>AAGVAAWLPFARAAAIGWMPVASGPMPAPPRQERKRTQDALIVLNVSGTRFQTWQDTLERYPDTLLGSSERDFFYHPETQQYFFDRDPDIFRHILNFYRTGKLHYPRHECISAYDEELAFFGLIPEIIGDCCYEEYKDRRRENAERLQDDADTDTAGESALPTMTARQRVWRAFENPHTSTMALVFYYVTGFFIAVSVIANVVETVPCGSSPGHIKELPCGERYAVAFFCLDTACVMIFTVEYLLRLAAAPSRYRFVRSVMSIIDVVAILPYYIGLVMTDNEDVSGAFVTLRVFRVFRIFKFSRHSQGLRILGYTLKSCASELGFLLFSLTMAIIIFATVMFYAEKGSSASKFTSIPAAFWYTIVTMTTLGYGDMVPKTIAGKIFGSICSLSGVLVIALPVPVIVSNFSRIYHQNQRADKRRAQKKARLARIRAAKSGSANAYMQSKRSGLLSNQLQSSEDEQAFVSKSGSSFETQHHHLLHCLEKTTNHEFVD[4x];>[2x]PEGLEQLEAQTNFTKRELQVLYRGFKNECPSGVVNEDTFKQIYAQFFPHGDASTYAHYLFNAFDTTQTGSVKFEDFVTALSILLRGTVHEKLRWTFNLYDINKDGYINKEEMMDIVKAIYDMMGKYTYPVLKEDTPRQHVDVFFQKMDKNKDGIVTLDEFLESCQEDDNIMRSLQLFQNVM;>[2x]EGLEQLEAQTNFTKRELQVLYRGFKNECPSGVVNEDTFK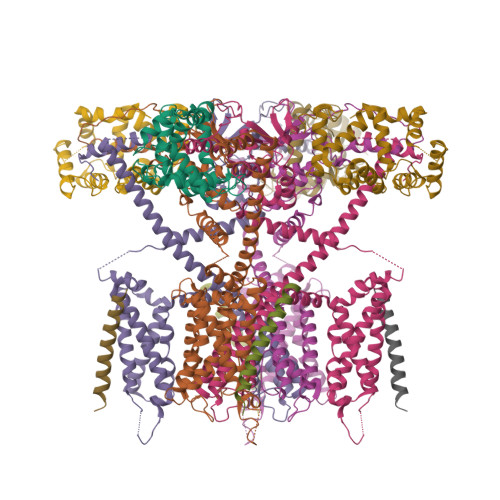QIYAQFFPHGDASTYAHYLFNAFDTTQTGSVKFEDFVTALSILLRGTVHEKLRWTFNLYDINKDGYINKEEMMDIVKAIYDMMGKYTYPVLKEDTPRQHVDVFFQKMDKNKDGIVTLDEFLESCQEDDNIMRSLQLFQNVM;>AAAAKGIAIALLVILVICSLIVTSVILLTPA[2x];>AKGIAIALLVILVICSLIVTSVILLTPA[2x]N-[3-[(4S)-2-azanyl-4-methyl-1,3-thiazin-4-yl]-4-fluoranyl-phenyl]-5-cyano-pyridine-2-carboxamide | C18 H14 F N5 O S | 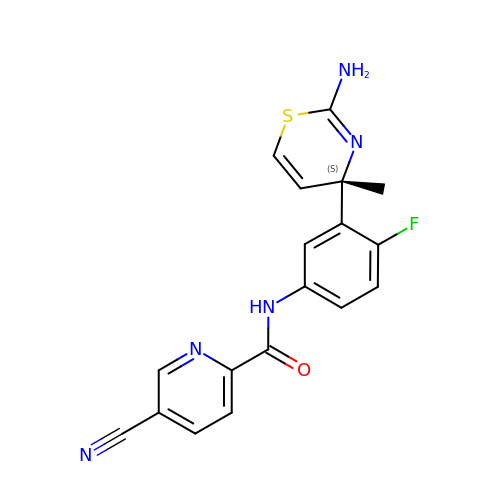VLLFGVHGKLDDLW-SFHVURJKSA-N> MGSSHHHHHHSQENLYFQGMVFSYEHYMNLLFHLDNSKETVPPEIAKRIISNAIAPVITVTSTPLFDKHIQETYKVDSLYMLLRFFGGCVSDRDQANEAKVGQHEHEVCDASDSTDSIPKNKNLEVPNLSKKGSRSRSNSLFQRDSTQSQYIRFTRPLGDLIETRDANDMLFNYHSLEVFLDNYLKLVAANTDEMVPHNLLKKSIYHSFFSLAISSTNNLSPYETFNHPILSLIALDISNGEVYEDARDLLVNFKNLNHNTENFPIFMNTNEMLPVFLLCYNDDSQEEFEKCQALAKKLKKQLFVESILLALWKDSFIYDENSVIQLHQPVMSSLEEILFFLQAPTQTTLSLALINSIYDMLDYLVYDLMIPFMKRKVSFWEETILQPRKSL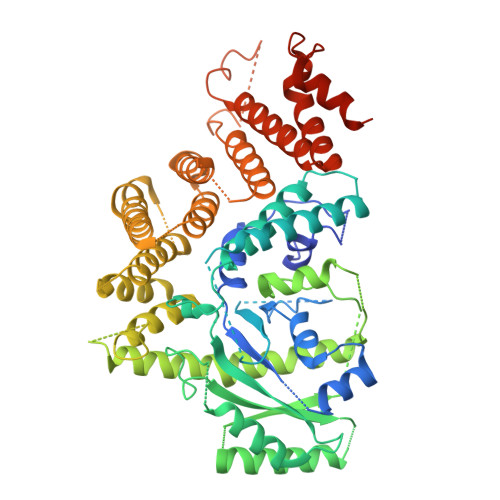FNGAKFFKKFMNKNPVNGNHQHNSLTRDSQGNEYFASSSSEFLMRKLADWSMMLSDFKTAYSTYESLMDDLDAFPKYLASCIEWCAVSLLMGAQSIVTVKMIKNDINPLIERALATYENCSRIQRGKGKESNSLDVTEPVRSYETRCMILASELFLSLSNTWTSTPYAIQYLETILDECKLGPCSQIMVWERLSDCYNLRVDPRIKHRVGAMKKDAKDTEDLRGEHKYSTDHFTDEDILSEGLTRRRKAAFFRLIAAKKWAEQKQWRQVSWCLKDIESTYSEIKFLHGNGLILSKLKNQLNLKDVDSAPRPSEKNLTRTSVSFIG> GSSMASGISVEELLKLAKAAYYSGTTVEEAYKLALKLGISVEELLKLAEAAYYSGTTVEEAYKLALKLGISVEELLKLAKAAYYSGTTVEEAYKLALKLGISVEELLKLAKAAYYSGTTVEEAYKLAL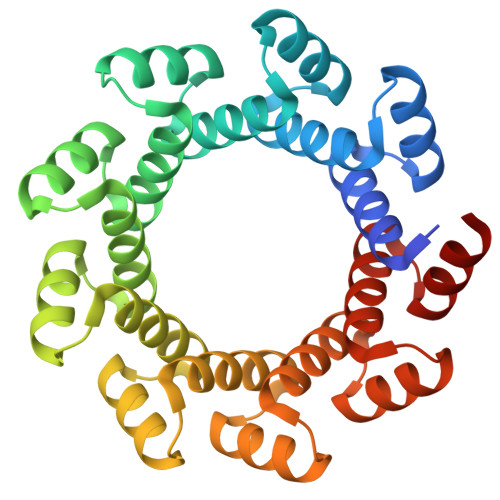KLGISVEELLKLAEAAYYSGTTVEEAYKLALKLGISVEELLKLAKAAYYSGTTVEEAYKLALKLGISVEELLKLAKAAYYSGTTVEEAYKLALKLGISVEELLKLAEAAYYSGTTVEEAYKLALKLGISVEELLKLAKAAYYSGTTVEEAYKLALKLG>SSRSFPEDDEPLNTVDYHYSRQYPVFRGRPSGNESQHRLDFQLMLKIRDTLYIAGRDQVYTVNLNDIPQTEVIPSKKLTWRSRQQDRENCAMKGKHKDECHNFIKVFVPRNDEMVFVCGTNAFNPMCRYYRLSTLEYDGEEISGLARCPFDARQTNVALFADGKLYSATVADFLASDAVIYRSMGDGSALRTIKYDSKWIKEPHFLHAIEYGNYVYFFFREIAVEHNNLGKAVYSRVARICKNDMGGSQRVLEKHWTSFLKARLNCSVPGDSFFYFDVLQSITDIIQINGIPTVIGVFTTQLNSIPGSAVCAFGMDDIEKVFKGRFKEQKTPDSVWTAVPEDKVPKPRPGCCAKHGLAEAYKTSIDFPDDTLSFIKSHPLMDSAVPPIADEPWFTKTRVRYRLTAIEVDRSAGPYQNYTVIFVGSEAGVVLKVLAKTSPFSLNDSVLLEEIEAYNPAKCSAESEEDRK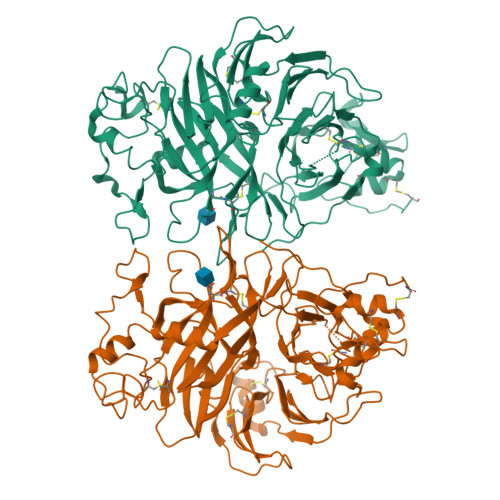VVSLQLDRDHHALYVAFSSCVVRIPLSRCERYGSCKKSCIASRDPYCGWLSQGVCERVTLGMLAGGYEQDTEYGNTAHLGDCHE[2x]> ADEPVWRSEQAIGAIAASQEDGVFVASGSCLDQLDYSLEHSLSRLYRDQAGNCTEPVSLAPPARPRPGSSFSKLLLPYREGAAGLGGLLLTGWTFDRGACEVRPLGNLSRNSLRNGTEVVSCHPQGSTAGVVYRAGRNNRWYLAVAATYVLPEPETASRCNPAASDHDTAIALKDTEGRSLATQELGRLKLCEGAGSLHFVDAFLWNGSIYFPYYPYNYTSGAATGWPSMARIAQSTEVLFQGQASLDCGHGHPDGRRLLLSSSLVEALDVWAGVFSAAAGEGQE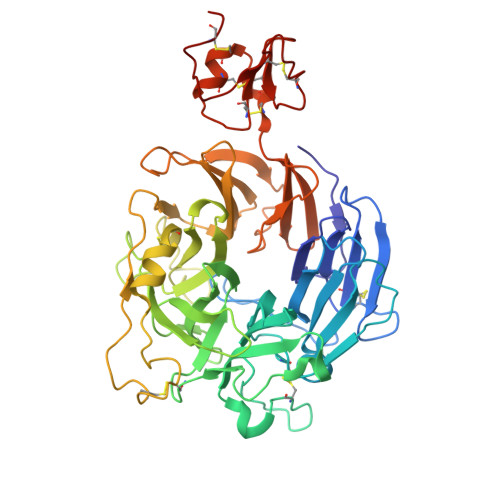RRSPTTTALCLFRMSEIQARAKRVSWDFKTAESHCKEGDQPERVQPIASSTLIHSDLTSVYGTVVMNRTVLFLGTGDGQLLKVILGENLTSNCPEVIYEIKEETPVFYKLVPDPVKNIYIYLTAGKEVRRIRVANCNKHKSCSECLTATDPHCGWCHSLQRCTFQGDCVHSENLENWLDISSGAKKCPGAP>MGHHHHHHHHHHSSGHIEGRHMPNDQTHPFRGVNALPFEERYDNFIGGEWVAPVSGRYFTNTTPITGAEIGQIARSEAGDIELALDAAHAAKEKWGATSPAERANIMLKIADRMERNLELLATAETWDNGKPIRETMAADLPLAIDHFRYFAGVLRAQEGSISQIDDDTVAYHFHEPLGVVGQIIPWNFPLLMACWKLAPAIAAGNCVVLKPAEQTPAGIMVWANLIGDLLPPGVLNIVNGFGLEAGKPLASSNRIAKIAFTGETTTGRLIMQYASENLIPVTLELGGKSPNIFFADVAREDDDFFDKALEGFTMFALNQGEVCTCPSRVLIQESIYDKFMERAVQRVQAIKQGDPRESDTMIGAQASSEQKEKILSYLDIGKKEGAEVLTGGKAADLGGELSGGYYIEPTIFRGNNKMRIFQEEIFGPVVSVTTFKDQAEALEIANDTLYGLGAGVWSRDANTCYRMGRGIKAGRVWTNCYHAYPAHAAFGGYKQSGIGRETHKMMLDHYQQTKNMLVSYSPKKLGFF[4x]

Here, we show that Paracoccus denitrificans assimilates ethylene glycol solely via NAD-dependent alcohol and aldehyde dehydrogenases. We report the functional and structural characterization of EtgB and EtgA, key enzymes encoded by this etg gene cluster. We hypothesized that the alcohol dehydrogenase EtgB can convert ethylene glycol into glycolaldehyde, which is subsequently further converted into glycolate by the aldehyde dehydrogenase EtgA. The cryo-EM structures of EtgA and EtgB, determined at 3.1 and 3.0 Å resolution, respectively, provide a detailed insight into the active site of these enzymes and a starting point for structure-guided mutagenesis.

Enzyme assays revealed that EtgA readily oxidizes glycolaldehyde, albeit with a 2.5-fold lower catalytic efficiency than acetaldehyde. In contrast, the inter-dimer contacts show energetically unfavorable ΔG values of +2.3 and +4.5 kcal/mol, consistent with weak contacts between the ‘dimer-of-dimers’, resulting in flexibility and a weak definition of the cryo-EM map. EtgA is structurally similar to other bacterial aldehyde dehydrogenases and has a canonical active site with catalytic Cys and Glu residues. The aldehyde dehydrogenase EtgA efficiently converts glycolaldehyde into glycolate, enabling the subsequent conversion of glycolate to glyoxylate, which then enters central carbon metabolism via the BHAC.>[3x]SVSENSGAAYGFAVKLP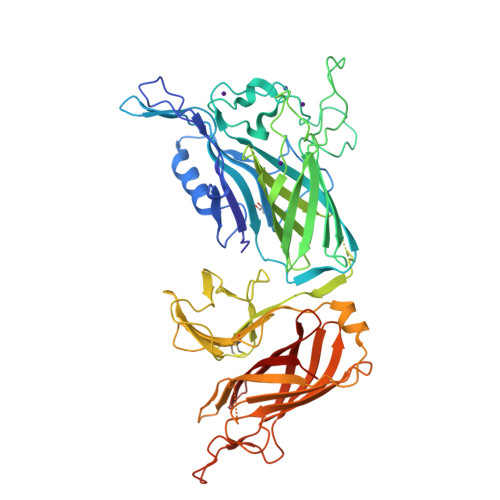RRNAHFNPKYKEKHKPLGSMDWKKLQRGEPNSFSERDELEKKRGSSELIESKWEDGQSRVVGYTNFTYVRSGYVYLNKNNIDIKNNIVLFGPDGYLYYKGKEPSKELPSEKITYKGTWDYVTDAMEKQRFEGLGSAAGGDKSGALSALEEGVLRNQAEASSGHTDFGMTSEFEVDFSDKTIKGTLYRNNRITQNNSENKQIKTTRYTIQATLHGNRFKGKALAADKGATNGSHPFISDSDSLEGGFYGPKGEELAGKFLSNDNKVAAVFGAKQKDKKDGENAAGPATETVIDAYRITGEEFKKEQIDSFGDVKKLLVDGVELSLLPSEGNKAAFQHEIEQNGVKATVCCSNLDYMSFGKLSKENKDDMFLQGVRTPVSDVAARTEANAKYRGTWYGYIANGTSWSGEASNQEGGNRAEFDVDFSTKKISGTLTAKDRTSPAFTITAMIKDNGFSGVAKTGENGFALDPQNTGNSHYTHIEATVSGGFYGKNAIEMGGSFSFPGNAPEGKQEKASVVFGAKRQQLVQ Fas-associated protein with death domain (FADD), procaspase-8, and cellular FLICE-inhibitory proteins (cFLIP) assemble through death-effector domains (DEDs), directing death receptor signaling towards cell survival or apoptosis. In this work, we present the crystal and cryo-EM structures of ternary FADD-Casp-8-cFLIP DED complexes, unveiling FADD-FADD, FADD-Casp-8, FADD-cFLIP, Casp-8-cFLIP, and cFLIP-cFLIP DED assemblies in a complex. The atomic coordinates depict how FADDDED and Casp-8tDED could assemble a helical 1:5 and 3:3 intermediate complexes, and how these FADD-Casp-8 intermediate complexes are targeted and capped by four cFLIPtDED molecules. The resultant helical Casp-8tDED-cFLIPtDED hetero-double layer appears to locally activate Casp-8.

We successfully reconstituted the ternary complex FADDFuL_H9G-Casp-8tDED_F122G/L123G-cFLIPtDED_H7G complex, henceforth referred to as the FAFuL_H9G-C8FGLG-CFH7G complex. Subsequently, we obtained the protein crystals and determined the crystal structure at 3.1 Å resolution using the MR-SAD method, in which FADD DD is not visible. Notably, the crystal structure reveals a 1:5:4 stoichiometry for the FAFuL_H9G-C8FGLG-CFH7G complex. This complex represents a single-FADD ternary DED complex, which fits the corresponding SAXS envelope. The single-FADD complex structure unveils additional FADDDED-Casp-8tDED assembly, in which Casp-8tDED assembles a type III-II-III CSS-mediated pentamer, containing Casp-8tDED molecules C8a, C8b, C8c, C8d, and C8e. Although the only FADDDED molecule FAl uses distinct surfaces to interact with three different Casp-8tDED molecules C8a, C8d, and C8e, these interfaces are too small, which are ~330 to ~500 Å2, to form 1:1 FADD-Casp-8 complexes for intermediate complex formation. Instead, the III-II-III CSS contributes larger interface areas, which are ~780 to ~820 Å2 corresponding to the buried surface area (the BSA) of ~1560 to ~1640 Å2, providing Casp-8tDED the ability to self-assemble transient oligomers. These oligomers then form a composite-binding site (CBS) with a larger interface area of 835 ~ 1,280 Å2 to interact effectively with FADD, promoting the formation of a FADD-Casp-8 intermediate complex. In the 1:5:4 FAFuL_H9G-C8FGLG-CFH7G complex structure, three Casp-8tDED molecules C8c, C8d, and C8a provide, respectively, a type Ia, a type IIa, and a type IIIa surfaces, while FADDDED molecule FAl provides a type IIa and a type IIIa surfaces to complete the CBS to recruit cFLIPtDED_H7G molecule CFk. In the single-FADD structure, the halt of Casp-8 filamentation at the upper end results from the inability of the CSS of Casp-8tDED molecule C8e to bind and stabilize another Casp-8 tDED when there’s no FADD in the adjoining space.

>[5x]MDFSRNLYDIGEQLDSEDLASLKFLSLDYIPQRKQEPIKDALMLFQRLQEKRMLEESNLSFLKELLFRINRLDLLITYLNTRKEEMERELQTPGRAQISAYRVMLYQISEEVSRSELRSFKGGLQEEISKCKLDDDMNLLDIFIEMEKRVILGEGKLDILKRVCAQINKSLLKIINDYEEFSKER;>[4x]MSAEVIGQVEEALDTDEKEMLLFLCRDVAIDVVPPNVRDLLDILRERGKLSVGDLAELLYRVRRFDLLKRILKMDRKAVETHLLRNPHLVSDYRVLMAEIGEDLDKSDVSSLIFLMKDYMGRGKISKEKSFLDLVVELEKLNLVAPDQLDLLEKCLKNIHRIDLKTKIQKYKQSVQGAGTS;> MDPFLVLLGSVSSSLSSSELTELKFLCLGRVGKRKLERVQSGLDLFSMLLEQNDLEPGHTELLRELLASLRRHDLLRRVDDFEAGAAAGAAPGEEDLCAAFNVICDNVGKDWRRLARQLKVSDTKIDSIEDRYPRNLTERVRESLRIWKNTEKENATVAHLVGALRSCQMNLVADLVQEVQQARDLQNRSGAMSPMSWNSDASTSEASLEHHHHHH>AARYDDILYFPASRYPETGAHISDAIKAGHSDVCTIERSGADKRRQESLKGIPTKPGFDRDEWPMAMCEEGGKGASVRYVSSSDNRGAGSWVG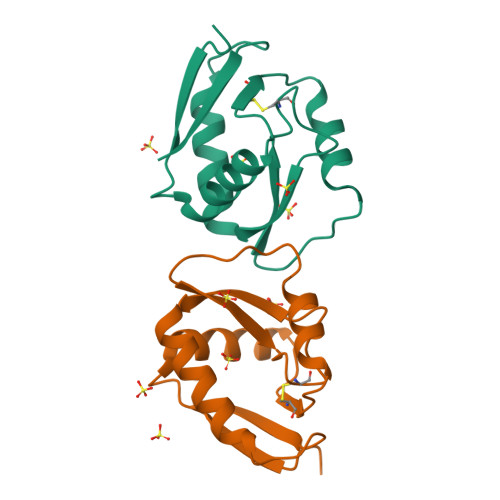NRLSGFADGTRILFIVQ[2x]> MALRDFCSVDGSDLFWEWNVTWNTSNPDFTKCFQNTVLVWVPCSYLWVCFPFYFLYLSHHDRGYIQMTHLNKAKTALGFLLWIVCWADLFYSFWERSMGKLLAPVFLVSPTLLGITMLLATFLIQIERRRGVQSSGIMLTFWLIALLCALAILRSKIMTALKEDARVDVFRDVTFYIYFSLVLIQLVLSCFSDRSPLFSETINDPNPCPESSASFLSRITFWWITGMMVQGYRQPLESTDLWSLNKEDTSEQVVPVLVKNWKKECAKSRKQPVKIVYSSKDPAKPKGSSKVDVNEEAEALIVKCPQKERDPSLFKVLYKTFGPYFLMSFLFKAVHDLMMFAGPEILKLLINFVNDKKAPEWQGYFYTALLFISACLQTLVLHQYFHICFVSGMRIKTAVIGAVYRKALVITNAARKSSTVGEIVNLMSVDAQRFMDLATYINMIWSAPLQVILALYLLWLNLGPSVLAGVAVMVLMVPLNAVMAMKTKTYQVAHMKSKDNRIKLMNEILNGIKVLKLYAWELAFKDKVLAIRQEELKVLKKSAYLAAVGTFTWVCTPFLVALSTFAVYVTVDENNILDAQKAFVSLALFNILRFPLNILPMVISSIVQASVSLKRLRVFLSHEDLDPDSIQRRPIKDAGATNSITVKNATFTWARNDPPTLHGITFSVPEGSLVAVVGQVGCGKSSLLSALLAEMDKVEGHVTVKGSVAYVPQQAWIQNISLRENILFGRQLQERYYKAVVEACALLPDLEILPSGDRTEIGEKGVNLSGGQKQRVSLARAVYCDSDVYLLDDPLSAVDAHVGKHIFENVIGPKGLLKNKTRLLVTHAISYLPQMDVIIVMS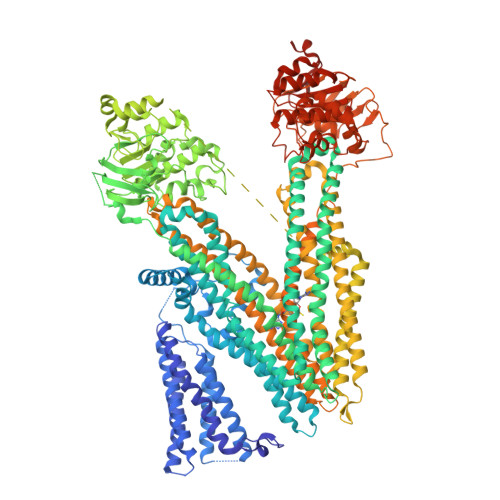GGKISEMGSYQELLARDGAFAEFLRTYASAEQEQGQPEDGLAGVGGPGKEVKQMENGMLVTDTAGKQMQRQLSSSSSYSRDVSQHHTSTAELRKPGPTEETWKLVEADKAQTGQVKLSVYWDYMKAIGLFISFLSIFLFLCNHVASLVSNYWLSLWTDDPIVNGTQEHTQVRLSVYGALGISQGITVFGYSMAVSIGGIFASRRLHLDLLHNVLRSPISFFERTPSGNLVNRFSKELDTVDSMIPQVIKMFMGSLFNVIGACIIILLATPMAAVIIPPLGLIYFFVQRFYVASSRQLKRLESVSRSPVYSHFNETLLGVSVIRAFEEQERFIRQSDLKVDENQKAYYPSIVANRWLAVRLECVGNCIVLFASLFAVISRHSLSAGLVGLSVSYSLQVTTYLNWLVRMSSEMETNIVAVERLKEYSETEKEAPWQIQDMAPPKDWPQVGRVEFRDYGLRYREDLDLVLKHINVTIDGGEKVGIVGRTGAGKSSLTLGLFRIKESAEGEIIIDDINIAKIGLHDLRFKITIIPQDPVLFSGSLRMNLDPFSQYSDEEVWTSLELAHLKGFVSALPDKLNHECAEGGENLSVGQRQLVCLARALLRKTKILVLDEATAAVDLETDDLIQSTIRTQFDDCTVLTIAHRLNTIMDYTRVIVLDKGEIQEWGSPSDLLQQRGLFYSMAKDSGLVKLGSENLYFQGGSGGSGHHHHHHHHHHH>[4x]HHHHHHGSEL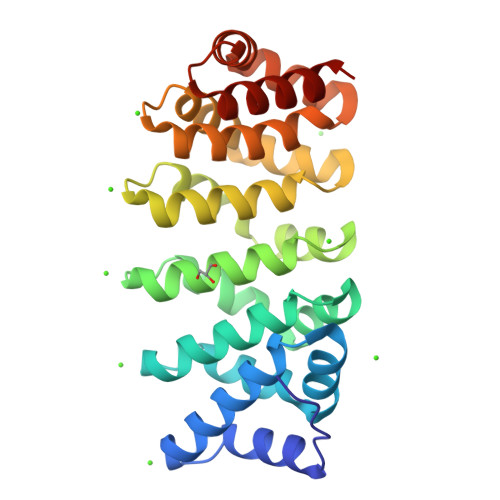PQMVQQLNSPDQQELQSALRKLSQIASGGDEQIQAVIDAGALPALVQLLSSPNEQILQEALWTLGNIASGGDEQIQAVIDAGALPALVQLLSSPNEQILQEALWTLGNIASGGDEQIQAVIDAGALPALVQLLSSPNEQILQEALWTLGNIASGGDEQIQAVIDAGALPALVQLLSSPNEQILQEALWTLGNIASGGNEQKQAVKEAGALEKLEQLQSHENEKIQKEAQEALEKLQS N-{[3,5-dibromo-2-(methoxymethoxy)phenyl]methyl}-2-nitrobenzamide | C16 H14 Br2 N2 O5 | 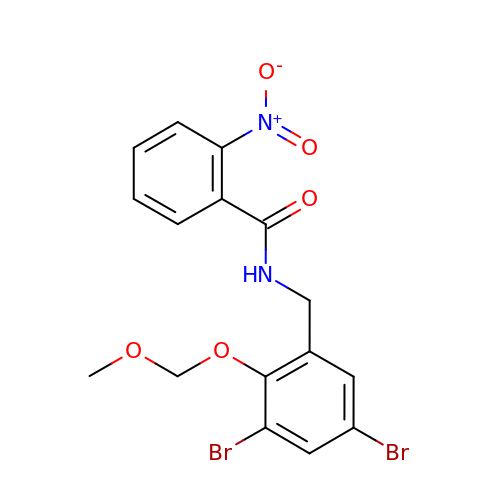ZLGSUAWZOLKSNW-UHFFFAOYSA-N>[2x]MRGSHHHHHHGSMGSLEKFNLIDEPWIPVLKGGRVVEVGIGEALLRAHEFARIETPSPLEEAVLHRLLLAVLHRALSGPRCPEDVLDWWRKGGFPQDPIRDYLNRFRDRFFLFHPEAPFLQVADLPEENPLPWSKLLPELASGNNPTLFDHTTEENLPKATYAQAARALLVHQAFAPGGLLRRYGVGSAKDAPVARPALFLPTGQNLLETLLLNLVPYTPEDDAPIWEVPPLRLGDLEGARTKWPLTGRTRVYTWPARGVRLLDEGDGVRFMGYGPGVEPLEATHRDPMVAQRLDAKGNLLVLRLSEERSFWRDFSAMLPRQGGKVAA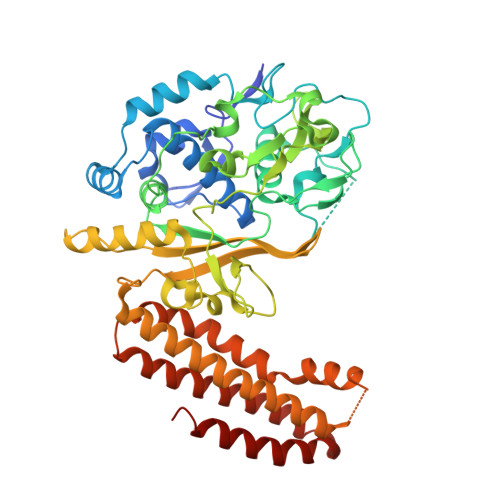TLEHAENLQGELEDEGLEGRITLRVLGQVSDQAKVLDIRREVYPLPSGLLTPKAEENLEKALKMAEELGQGLKHLAQEVAKAVVGERDRGHGRSPYLEELTKLANSLPLERLYWHALDGAFPRFFARVEEEASLDLWREALRGAALEAWKATRRFLGTGARHLKALAQGEQEFGRLLGELGEEVRT>[2x]MPQPIHLKDHEKDARLVRRRVIVGAVAVVLLTLVLVARMYHLQVTQYEYHSTLSENNRVHVQPIPPTRGIIFDRNGVIIADNRPSFSLTITRERTEDLQKTLDTLVEILGLTEDDRAIFEKRMKQGRRPFEPVPIMFELNEEQIARIAVNQFRLPGVDVATQFVRHYPLKEHFAHSVGYVGRINEQELKNLDPINYSGTHHIGKTGIERFYESELHGTVGYEEVETNARGRVLRVLKRTDPIPGKDIVLSIDSRLQEAAENALAGRRGAIVAIQPSTGDVLAMVSQPSYDPNLFVTGISFKAYAELRDSIDRPLYNRVLRGLYPPGSTVKPAVALAGLDAGVVTPTSRVFDPGYYQLPNY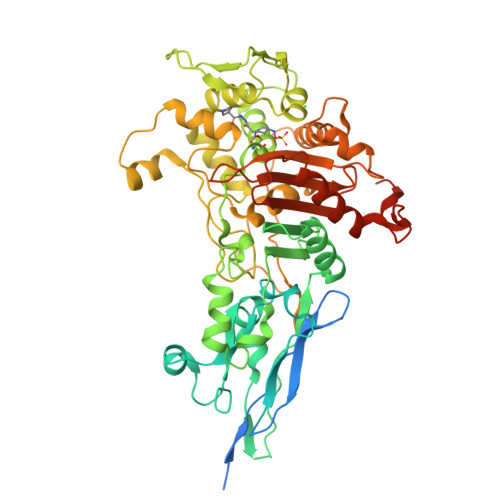DHKYRNWNRYGDGWVSLESAIYRSNDTYFYDLAHKLGIDRLHAFMSRFGFGQKVALDMFGEADGLMPSREWKRKTRRQVWYPGETLILGIGQGYMQATPIQLAQMTALLANKGHWIRPHLAKTIDGQPPVDPDPMPDIVLRDPANWDRVDYGMQQVVHGARGTARKVGATSAYLIAGKSGTAQVVAIKQNERYDRSKLLERHRDHALFVGFAPANNPQIAVAVMVENGESGSGVAAPVVKQVMDAWLLDEHGKLKAEYAEPVAPLAAAVAKPEPTAAEPEAPALEQ> EADLALGKAVFDGNCAACHAGGGNNVIPDHTLQKAAIEQFLDGGFNIEAIVYQ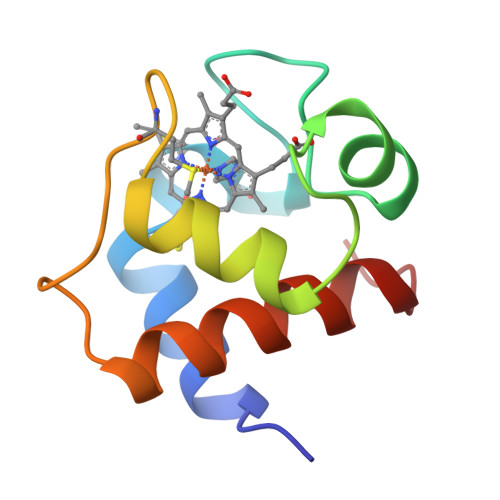IENGKGAMPAWDGRLDEDEIAGVAAYVYDQAAGNKW> MTDVQCEPALAGRKPKWADADIAELVDERTGRLDPRIYTDEALYEQELERIFGRSWLLMGHETQIPKAGDFMTNYMGEDPVMVVRQKNGEIRVFLNQCRHRGMRICRADGGNAKSFTCSYHGWAYDTGGNLVSVPFEEQAFPGLRKEDWGPLQARVETYKGLIFANWDADAPDLDTYLGEAKFYMDHMLDRTEAGTEAIPGIQKWVIPCNWKFAAEQFCSDMYHAGTTSHLSGILAGLPDGVDLSELAPPTEGI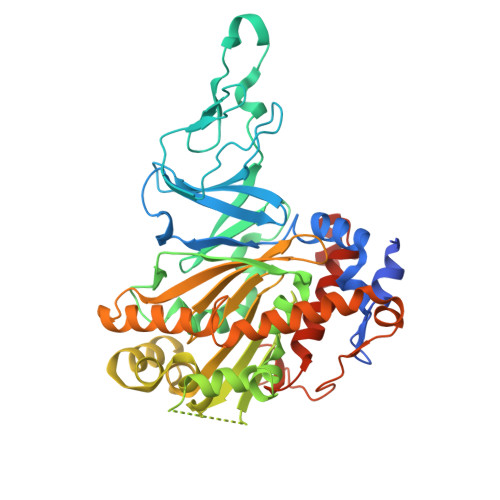QYRATWGGHGSGFYIGDPNLLLAIMGPKVTEYWTQGPAAEKASERLGSTERGQQLMAQHMTIFPTCSFLPGINTIRAWHPRGPNEIEVWAFTVVDADAPEEMKEEYRQQTLRTFSAGGVFEQDDGENWVEIQQVLRGHKARSRPFNAEMGLGQTDSDNPDYPGTISYVYSEEAARGLYTQWVRMMTSPDWAALDATRPAVSESTHT> G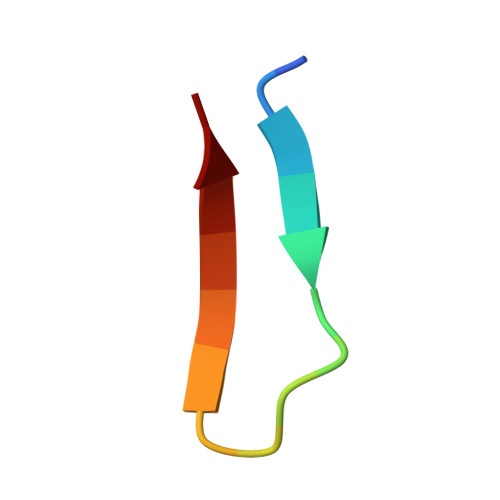PKWVKTDSDFIVLEI> PSAEECGYSDRVRSLTLGNSTITT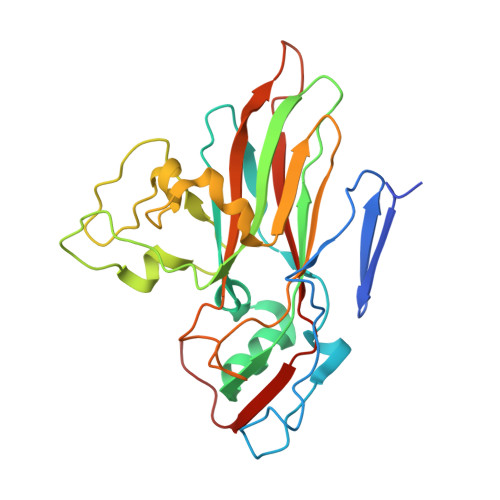QESANVVVGYGRWPEYLRDDEATAEDQPTQPDVATCRFYTLESVQWEKNSAGWWWKFPEALKDMGLFGQNMLYHYLGRAGYTIHVQCNASKFHQGCLLVVCVPEAEMGCSQTDKEVAAMNLTKGEAAHKFEPTKTNGEHTVQSIVCNAGMGVGVGNLTIYPHQWINLRTNNCATIVMPYVNSVPMDNMFRHYNFTLMVIPFAPLDYAAQASEYVPVTVTIAPMCAEYNGLRLAYQQ> FNLDAEAPAVLSGPPGSFFGFSVEFYRPGTD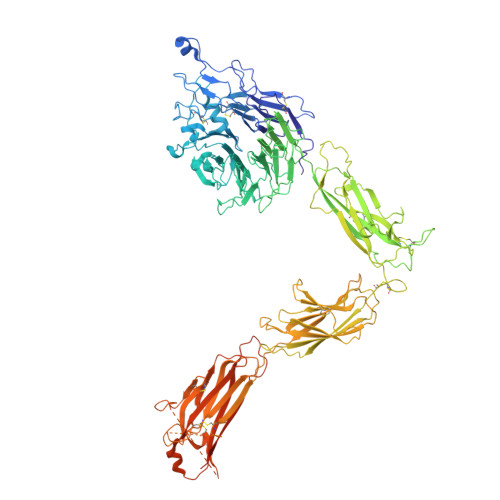GVSVLVGAPKANTSQPGVLQGGAVYLCPWGASPTQCTPIEFDSKGSRLLESSLSSSEGEEPVEYKSLQWFGATVRAHGSSILACAPLYSWRTEKEPLSDPVGTCYLSTDNFTRILEYAPCRSDFSWAAGQGYCQGGFSAEFTKTGRVVLGGPGSYFWQGQILSATQEQIAESYYPEYLINLVQGQLQTRQASSIYDDSYLGYSVAVGEFSGDDTEDFVAGVPKGNLTYGYVTILNGSDIRSLYNFSGEQMASYFGYAVAATDVNGDGLDDLLVGAPLLMDRTPDGRPQEVGRVYVYLQHPAGIEPTPTLTLTGHDEFGRFGSSLTPLGDLDQDGYNDVAIGAPFGGETQQGVVFVFPGGPGGLGSKPSQVLQPLWAASHTPDFFGSALRGGRDLDGNGYPDLIVGSFGVDKAVVYRGRPIVSASASLTIFPAMFNPEERSCSLEGNPVACINLSFCLNASGKHVADSIGFTVELQLDWQKQKGGVRRALFLASRQATLTQTLLIQNGAREDCREMKIYLRNESEFRDKLSPIHIALNFSLDPQAPVDSHGLRPALHYQSKSRIEDKAQILLDCGEDNICVPDLQLEVFGEQNHVYLGDKNALNLTFHAQNVGEGGAYEAELRVTAPPEAEYSGLVRHPGNFSSLSCDYFAVNQSRLLVCDLGNPMKAGASLWGGLRFTVPHLRDTKKTIQFDFQILSKNLNNSQSDVVSFRLSVEAQAQVTLNGVSKPEAVLFPVSDWHPRDQPQKEEDLGPAVHHVYELINQGPSSISQGVLELSCPQALEGQQLLYVTRVTGLNCTTNHPINPKGLELDPEGSLHHQQKREAPSRSSASSGPQILKCPEAECFRLRCELGPLHQQESQSLQLHFRVWAKTFLQREHQPFSLQCEAVYKALKMPYRILPRQLPQKERQVATAVQWTKAEGSYGVPLWIIILAILFGLLLLGLLIYILYKLGFFKRSLPYGTAMEKAQLKPPATSDA Quinol-dependent nitric oxide reductases (qNORs) are membrane-integrated, iron-containing enzymes of the denitrification pathway, which catalyze the reduction of nitric oxide (NO) to the major ozone destroying gas nitrous oxide (N2O). NORs catalyze the reduction of two molecules of nitric oxide (NO) to nitrous oxide (N2O), using two protons and two electrons to cleave the N─O bond and concurrent N─N bond formation: 2NO + 2H+ + 2e− → N2O + H2O. In contrast, qNORs are single subunit enzymes (NorZ), in which electrons are supplied by menaquinol. qNORs are found not only in denitrifying organisms but also in various pathogenic species, many of which lack the full denitrifying apparatus, bringing to attention the role of qNORs in detoxification. Cryo-EM structures unexpectedly revealed AxqNOR to be a dimer.

One of the mutants, Val495Ala, revealed an enhanced activity (by twofold) compared to wild type and was thus chosen for cryo-EM structure determination. A total of 227,000 particles were used in the final refinement (C2 symmetry), with a global resolution of 3.3 Å and a local resolution at 3.2 Å. The Val495Ala mutation appears to have increased conformational flexibility of Glu494. However, the overall structure of Val495Ala-BRIL is largely similar to that of the wild type, with some additional density between the dimer interface assigned as detergent molecules, which were used in solubilization [dodecyl maltoside (DDM)]. Density, which appeared to be phospholipid-like, was also seen near the dimer interface, with one phosphatidylethanolamine molecule providing an anchor between TMHII of one molecule and surrounding helices of the other molecule through Phe598 and Phe680. As a result of the improved resolution of the structure of the Val495Ala mutant, several new features could be resolved; most notably, a number of water molecules lining the polar channel from the cytoplasmic side to the binuclear site could be seen. A closer examination of a residue near the proposed proton entry site (Arg255) reveals a water molecule between Glu572 and Arg255, which may act as a proton entry point. A water molecule was found ligating the carboxyl group of Glu490 and Glu559 (the higher-resolution AxqNOR-Val495Ala structure provides clear density of Glu559), which is not the case in GsqNOR, as this water does not ligate to the equivalent residues Glu512 and Glu581. The significantly enhanced activity of Val495Ala is likely to arise from alleviating proton transfer as the rate-limiting step. This most likely results from increased conformational dynamics of Glu494, which shuttles the proton toward the catalytic pocket.

>[2x]MGPYRRLWFTLIAVLAVTFALLGFYGGEVYRQAPPIPEEVASADGTRLFGRDDILDGQTAWQSIGGMQLGSIWGHGAYQAPDWTADWLHRELMAWLDLAARDAHGRDYGQLDAPAQAALREQLKAEYRANRADAAGGKLTLSPRRAQAVAQTEAYYDQLFSDAPALHRSRENYAMKENTLPDANRRRQMTHFFFWTAWAAGTEREGTSVTYTNNWPHEPLIGNHPSSENVMWSIISVVVLLAGIGLLIWAWAFLRGKEEDEPPAPARDPLTTFALTPSQRALGKYLFLVVALFGFQVLLGGFTAHYTVEGQKFYGIDLSQWFPYSLVRTWHIQSALFWIATGFLAAGLFLAPLINGGRDPKYQKAGVDILFWALVLVVVGSFAGNYLAIAQIMPPDLNFWLGHQGYEYVDLGRLWQIGKFAGICFWLVLMLRGIVPALRTPGGDKNLLALLTASVGAIGLFYGAGFFYGERTHLTVMEYWRWWIVHLWVEGFFEAFATTALAFIFSTLGLVSRRMATTASLASASLFMLGGIPGTFHHLYFAGTTTPVMAVGASFSALEVVPLIVLGHEAWENWRLKTRAPWMENLKWPLMCFVAVAFWNMLGAGVFGFMINPPVSLYYIQGLNTTPVHAHAALFGVYGFLALGFTLLVLRYIRPQYALSPGLMKLAFWGLNLGLALMIFTSLLPIGLIQFHASVSEGMWYARSEAFMQQDILKTLRWGRTFGDVVFLLGALAMVVQVILGLLSGK> MDLAPDRATGRPWLPLHTLSVSQLLRVFWLLSLLPGQAWVHGAEPRQVFQVLEEQPPGTLVGTIQTRPGFTYRLSESHALFAINSSTGALYTTSTIDRESLPSDVINLVVLSSAPTYPTEVRVLVRDLNDNAPVFPDPSIVVTFKEDSSSGRQVILDTATDSDIGSNGVDHRSYRIIRGNEAGRFRLDITLNPSGEGAFLHLVSKGGLDREVTPQYQLLVEVEDKGEPKRRGYLQVNVTVQDINDNPPVFGSSHYQAGVPEDAVVGSSVLQVAAADADEGTNADIRYRLQDEGTPFQMDPETGLITVREPLDFEARRQYSLTVQAMDRGVPSLTGRAEALIQLLDVNDNDPVVKFRYFPATSRYASVDENAQVGTVVALLTVTDADSPAANGNISVQILGGNEQRHFEVQSSKVPNLSLIKVASALDRERIPSYNLTV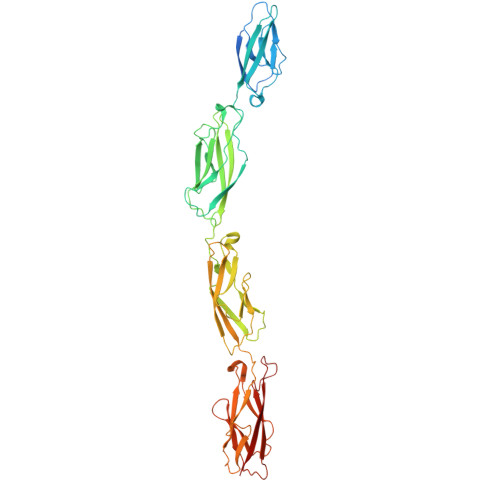SVSDNYGAPPGAAVQARSSVASLVIFVND>MAEKVLVTGGAGYIGSHTVLELLEAGYLPVVIDNFHNAFRGGGSLPESLRRVQELTGRSVEFEEMDILDQGALQRLFKKYSFMAVIHFAGLKAVGESVQKPLDYYRVNLTGTIQLLEIMKAHGVKNLVFSSSATVYGNPQYLPLDEAHPTGGCTNPYGKSKFFIEEMIRDLCQADKTWNAVLLRY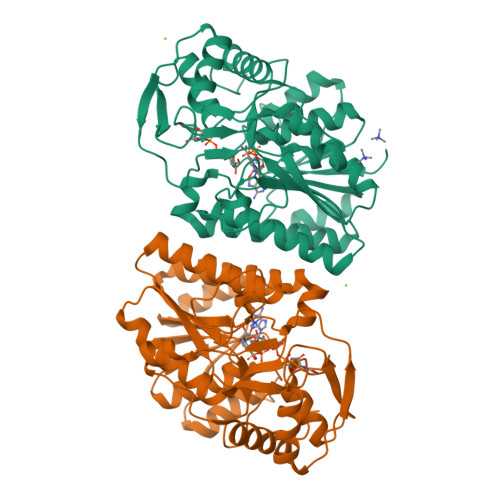FNPTGAHASGCIGEDPQGIPNNLMPYVSQVAIGRREALNVFGNDYDTEDGTGVRDYIHVVDLAKGHIAALRKLKEQCGCRIYNLGTGTGYSVLQMVQAMEKASGKKIPYKVVARREGDVAACYANPSLAQEELGWTAALGLDRMCEDLWRWQKQNPSGFGTQA[2x]>[4x]GAMGSEKSPSAQELKEQGNRLFVGRKYPEAAACYGRAITRNPLVAVYYTNRALCYLKMQQHEQALADCRRALELDGQSVKAHFFLG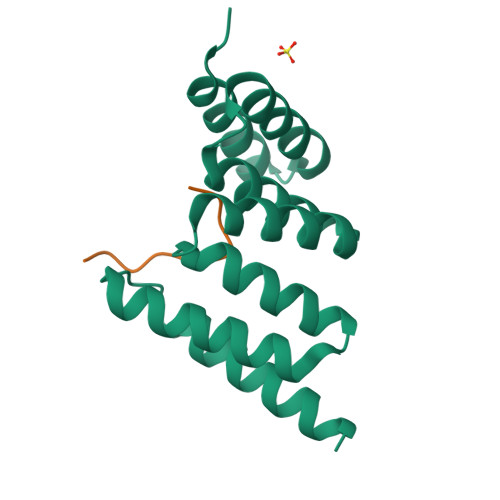QCQLEMESYDEAIANLQRAYSLAKEQRLNFGDDIPSALRIAKKKRWNSIEERR;>[4x]EFLPKTPIFRPD> MGSSHHHHHHSSGLVPRGSHMSSSRSSSMDKTGWITHCFGRFLIDLPPDAVINAGYYLWGDRIEYLDDKPTELAARVDRLEQEWRTQRHKSKGNMFLRKIDFGNESVGLLSWSSEVASKTYLLDTYVTSKPTWHVYRWKGKVSVDREQHAVEISRALARNLRSRAPKEIPSEPGFCIDHAYIAGDSFQVERFGVGVTFPEHPGARFEFRSSTGAELNSLLERVDGFVQNMLSTFAGMETLRKGKHPVG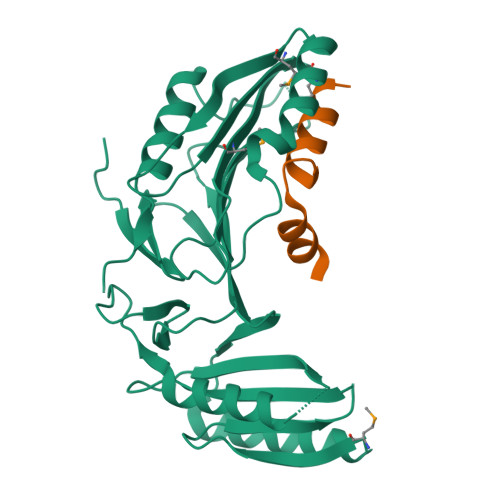SLPGEEYLVAGSDKGQRGYTFMWEVQGKEESLTEPNLTAGLAVLERSNENGKPPPPAFKSDKEALELWDTIVDSIRVRPTSSSPRGGNAGPSPAPKPATPGGQTLGDHYVYEEFLSSLKPKDSWLDDL;> DDLFASIGALWTWAWRGPKARQELLKA5'-O-[(R)-hydroxy(propanoylamino)phosphoryl]adenosine 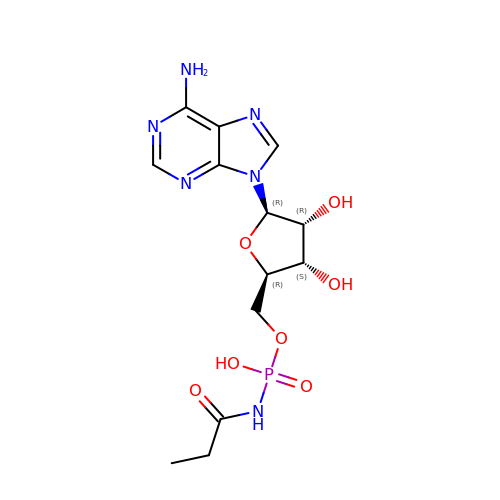| C13 H19 N6 O7 P | YXHIVTXRAWARSD-ZRFIDHNTSA-N>[2x]MHHHHHHGSENLYFQGSKFSAKRLPSTRLGTFLENRVNDFLRRQNHPESGEVTVRVVHASDKTVEVKPGMKARFVDSGEMAESFPYRTKALFAFEEIDGVDLCFFGMHVQEYGSDCPPPNQRRVYISYLDSVHFFRPKCLRTAVYHEILIGYLEYVKKLGYTTGHIWACPPS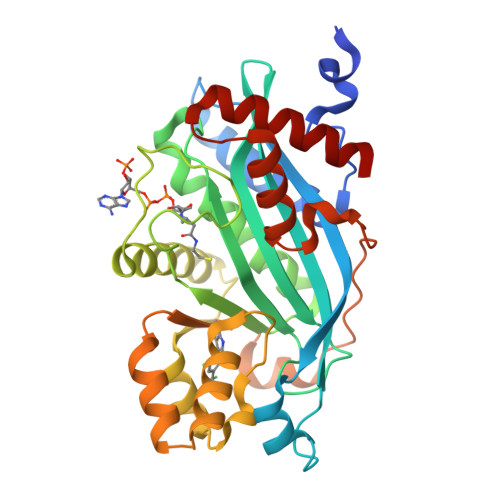EGDDYIFHCHPPDQKIPKPKRLQEWFKKMLDKAVSERIVHDYKDIFKQATEDRLTSAKELPYFEGDFWPNVLEESIKESGGSGSQKLYATMEKHKEVFFVIRLIAGPAANSLPPIVDPDPLIPCDLMDGRDAFLTLARDKHLEFSSLRRAQWSTMCMLVELHTQSQ> MGAEIPKELLRAQTNVILLNVLKQGDNYVYGIIKQVKEASNGEMELNEATLYTIFDRLEQDGIISSYWGDESQGG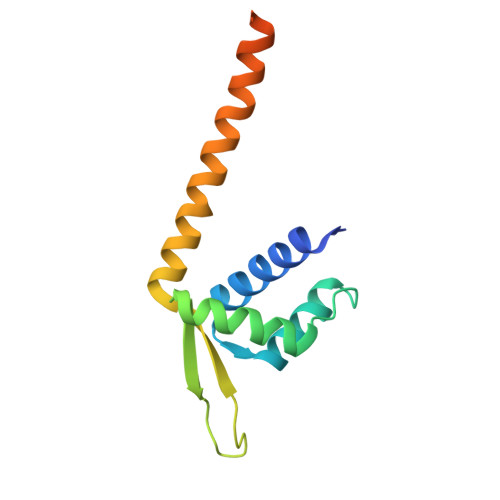RRKYYRLTEIGHENMRLAXESLSRVDKIIENLEANKKSEAIKSRGGSGGWSHPQFEK>[2x]AASSLDE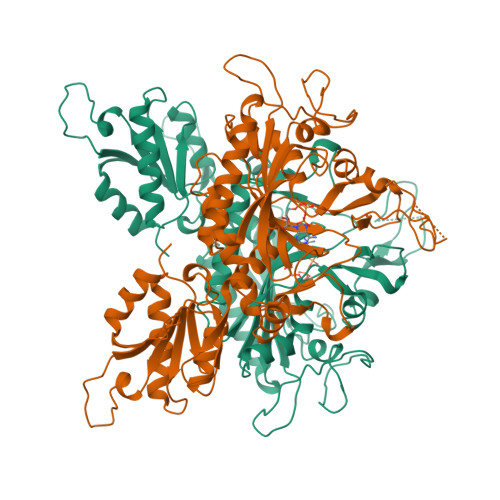LVALCKRRGFIFQSSEIYGGLQGVYDYGPLGVELKNNLKQAWWRRNVYERDDMEGLDASVLTHRLVLHYSGHEATFADPMVDNAKARYWTPPRYFNMMFQDLRGPRGGRGLLAYLRPETAQGIFVNFKNVLDATSRKLGFGIAQIGKAFRNEITPRNFIFRVREFEQMEIEYFVRPGEDEYWHRYWVEERLKWWQEMGLSRENLVPYQQPPESSAHYAKATVDILYRFPHGSLELEGIAQRTDFDLGSHTKDQEALGITARVLRNEHSTQRLAYRDPETGKWFVPYVIEPSAGVDRGVLALLAEAFTREELPNGEERIVLKLKPQLAPIKVAVIPLVKNRPEITEYAKRLKARLLALGLGRVLYEDTGNIGKAYRRHDEVGTPFAVTVDYDTIGQSKDGTTRLKDTVTVRDRDTMEQIRLHVDELEGFLRERLRW> GCRTTASLNITDGINVGEILANETSFSKSVVFTGISCDTSTDKIVYKNIQSDWVEVGPFGNGEKLKVKIESLGKTSDTIGKSSNAQAVLPYVVKIARGTPDFTGERKSTWFI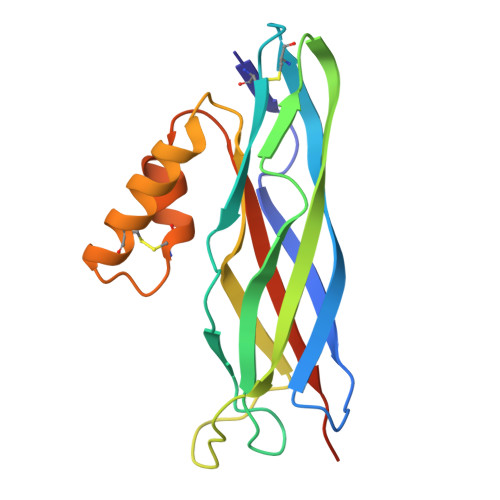SDTVIANIGGESSSSIDFWLGICKALKFNWCVNYLTSKLAGDTFTLGLNISYYPKNTTHHHHHH> AYKVTLKTPDGDITFDVEPGERLIDIGSEKADLPLSCQAGACSTCLGKIVSGTVDQSEGSFLDDEQIEQ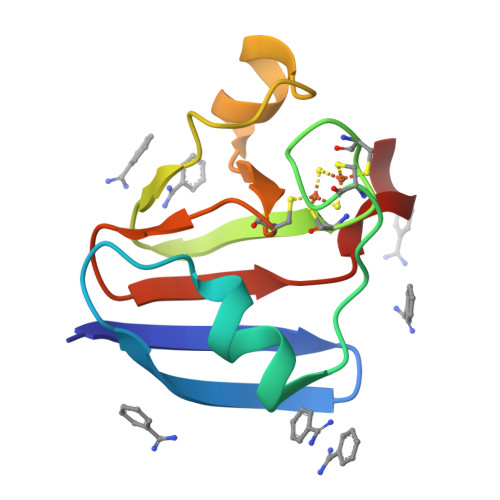GYVLTCIAIPESDVVIETHKEDEL> GSHMKNSVSVDLPGSMKVLVSKSSNADGKYDLIATVDALELSGTSDKNNGSGVLEGVKADASKVKLTISDDLGQTTLEVFKSDGSTLVSKKVTSNGSSTEEKIIIDGIIIEKIITRADGTRLEYTGIKSDGSGKAKEVLKGYVLEGTLTAE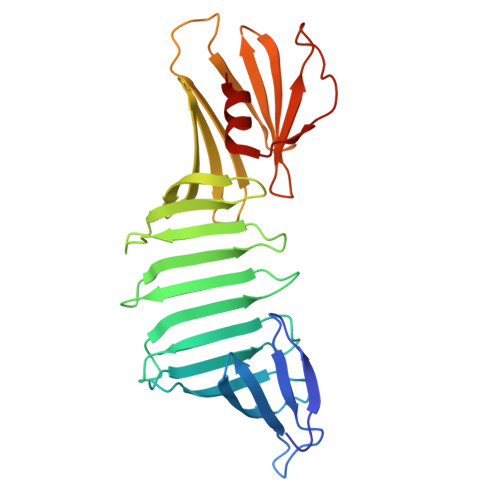KTTLVVKEGTVTLSKNISKSGEVSVELNDTDSSAATKKTAAWNSGTSTLTITVNSKKTKDLVFTSSNTITVQQYDSNGTSLEGSAVEITKLDEIKNALK> GEIQWVKPNKETGRLSINGPTRTKLEPSVFHDVFEGNKEPAVLHSKDPRLEVDFEQALFSKYVGNTLYEPDEYIKEAALHYANQLKQLEINTSQMSMEEACYGTENLEAIDLHTSAGYPYSALGIKKRDILDPTTRDVSKMKFYMDKYGLDLPYSTYVKDELRSIDKIKKGKSRLIEASSLNDSVY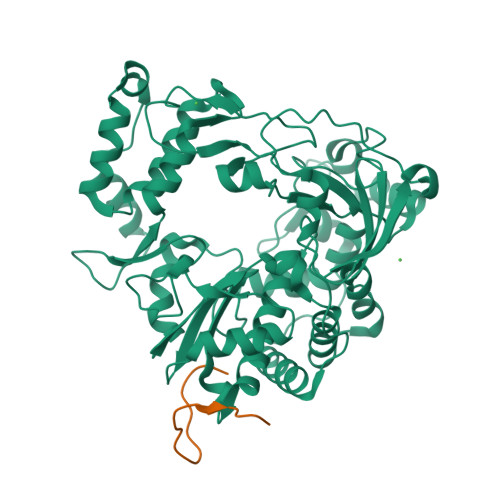LRMAFGHLYETFHANPGTITGSAVGCNPDTFWSKLPILLPGSLFAFDYSGYDASLSPVWFRALELVLREIGYSEEAISLIEGINHTHHVYRNKTYCVLGGMPSGCSGTSIFNSMINNIIIRALLIKTFKGIDLDELNMVAYGDDVLASYPFPIDCLELAKTGKEYGLTMTPADKSPCFNEVNWDNATFLKRGFLPDEQFPFLIHPTMPMREIHESIRWTKDARNTQDHVRSLCLLAWHNGKQEYEKFVSTIRSVPVGRALAIPNYENLRRNWLELF;> GAYSGAPKQVLKKPALRTATVQ> MIIGVLAIQGDVEEHEEAIKKAGYEAKKVKRVEDLEGIDALIIPGGESTAIGKLMKKYGLLEKIKNSNLPILGTCAGMVLLSKGTGINQILLELMDITVKRNAYGRQVDSFEKEIEFKDLGKVYGVFIRAPVVDKILSDDVEVIARDGDKI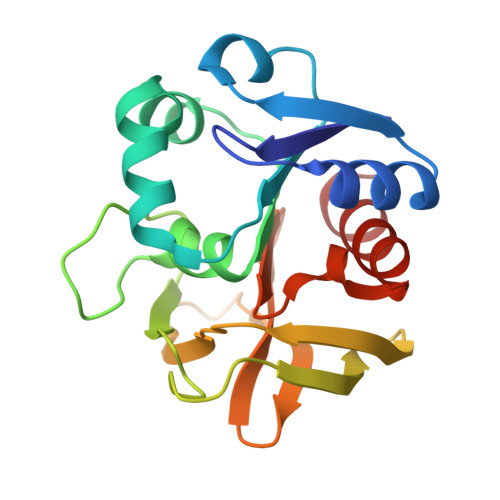VGVKQGKYMALSFHPELSEDGYKVYKYFVENCVKK>MSFFHASQRDALNQSLAEVQGQINVSFEFFPPRTSEMEQTLWNSIDRLSSLKPKFVSVTYGANSGERDRTHSIIKGIKDRTGLEAAPHLTCIDATPDELRTIARDYWNNGIRHIVALRGDLPPGSGKPEMYASDLVTLLKEVADFDISVAAYPEVHPEAKSAQADLLNLKRKVDAGVNRAITQFFFDVESYLRFRDRCVSAGIDVEIIPGILPVSNFKQAKKFADMTNVRIPAWMAQMFDGLDDDAETRKLVGANIAMDMVKILSREGVKDFHFYTLNRAEMSYAICHTLGVRPGLLEHH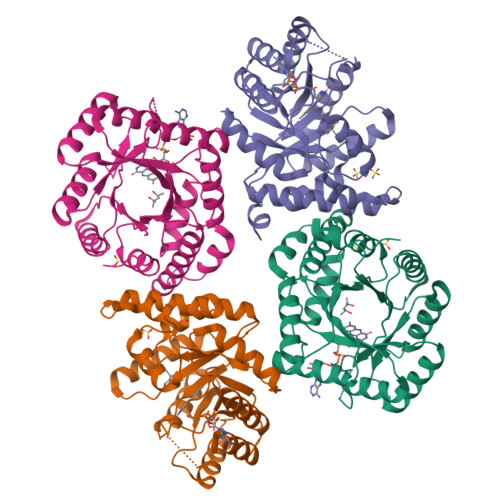HHHH[3x]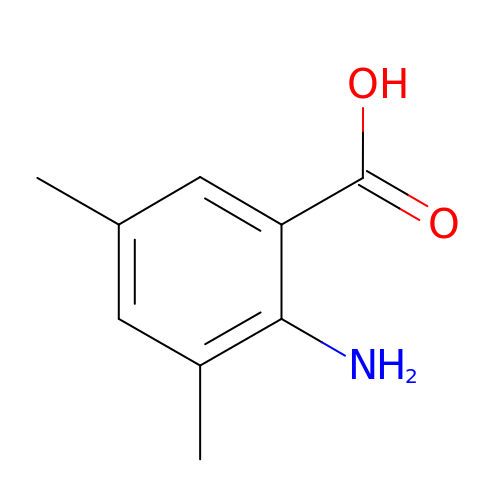2-amino-3,5-dimethylbenzoic acid | C9 H11 N O2 | GIMYRAQQQBFFFJ-UHFFFAOYSA-N(3R,5R)-7-{2-[(4-fluorobenzyl)carbamoyl]-4-(4-fluorophenyl)-1-(1-methylethyl)-1H-imidazol-5-yl}-3,5-dihydroxyheptanoic 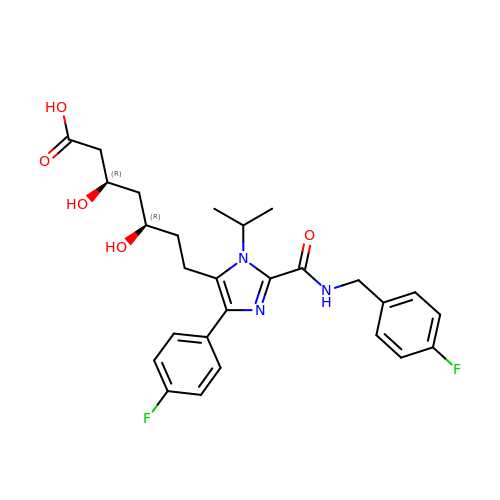acid | C27 H31 F2 N3 O5 | KNKKPGAQSAHIHV-FGZHOGPDSA-N>MRGSHHHHHHGMASELALMKITNPVLKGFNPDPSICRVGEDYYMAVSTFEWFPGVQIYHSKDLVHWRLAARPLQKTSQLDMKGNPDSGGVWAPCLSYADGQFWLIYSDIKVVDGPFKDGHNYLVTASEVDGDWSEPILLNSSGFDPSLFHDHSGKKYVLNMLWDHREKHHSFAGIALQEYSVAEKKLIGQRKVIFKGTPIKLTEAPHLYHIGDYYYLLTAEGGTRYEHAATIARSSHIEGPYEVHPDNPIVSAFHVPEHPLQKCGHASIVQTHTNEWYLAHLTGRPIQSSKESIFQ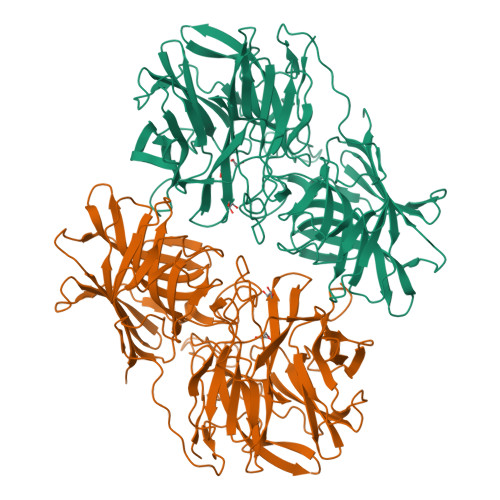QRGWCPLGRETAIQKLEWKDGWPYVVGGKEGTLEVEAPKIEEKVFAPTYHTVDEFKESTLNRHFQTLRIPFTDQIGSLTEKPQHLRLFGRESLTSKFTQAFVARRWQSFYFEAETAVSFFPENFQQAAGLVNYYNTENWTALQVTYDEELGRTLELSVCQNLAFSQPLTHKIIIPDEVTYVYLKVTVRKETYKYSYSFDQKEWKEIDVPFESIHLSDDFIRGGGFFTGAFVGMQCQDTSGERLPADFHYFRYEETDE[2x]> GAASMTQFEGFTNL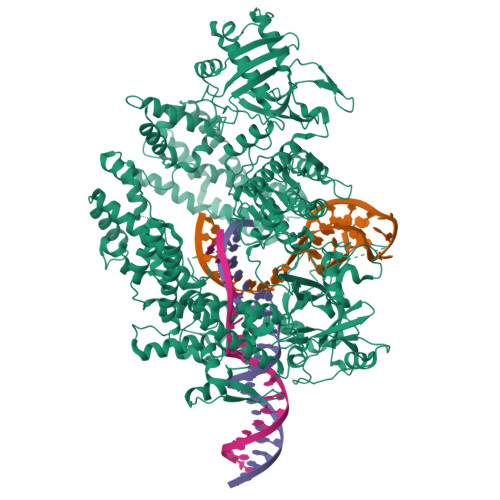YQVSKTLRFELIPQGKTLKHIQEQGFIEEDKARNDHYKELKPIIDRIYKTYADQCLQLVQLDWENLSAAIDSYRKEKTEETRNALIEEQATYRNAIHDYFIGRTDNLTDAINKRHAEIYKGLFKAELFNGKVLKQLGTVTTTEHENALLRSFDKFTTYFSGFYENRKNVFSAEDISTAIPHRIVQDNFPKFKENCHIFTRLITAVPSLREHFENVKKAIGIFVSTSIEEVFSFPFYNQLLTQTQIDLYNQLLGGISREAGTEKIKGLNEVLNLAIQKNDETAHIIASLPHRFIPLFKQILSDRNTLSFILEEFKSDEEVIQSFCKYKTLLRNENVLETAEALFNELNSIDLTHIFISHKKLETISSALCDHWDTLRNALYERRISELTGKITKSAKEKVQRSLKHEDINLQEIISAAGKELSEAFKQKTSEILSHAHAALDQPLPTTLKKQEEKEILKSQLDSLLGLYHLLDWFAVDESNEVDPEFSARLTGIKLEMEPSLSFYNKARNYATKKPYSVEKFKLNFQMPTLASGWDVNKEKNNGAILFVKNGLYYLGIMPKQKGRYKALSFEPTEKTSEGFDKMYYDYFPDAAKMIPKCSTQLKAVTAHFQTHTTPILLSNNFIEPLEITKEIYDLNNPEKEPKKFQTAYAKKTGDQKGYREALCKWIDFTRDFLSKYTKTTSIDLSSLRPSSQYKDLGEYYAELNPLLYHISFQRIAEKEIMDAVETGKLYLFQIYNKDFAKGHHGKPNLHTLYWTGLFSPENLAKTSIKLNGQAELFYRPKSRMKRMAHRLGEKMLNKKLKDQKTPIPDTLYQELYDYVNHRLSHDLSDEARALLPNVITKEVSHEIIKDRRFTSDKFFFHVPITLNYQAANSPSKFNQRVNAYLKEHPETPIIGIDRGERNLIYITVIDSTGKILEQRSLNTIQQFDYQKKLDNREKERVAARQAWSVVGTIKDLKQGYLSQVIHEIVDLMIHYQAVVVLENLNFGFKSKRTGIAEKAVYQQFEKMLIDKLNCLVLKDYPAEKVGGVLNPYQLTDQFTSFAKMGTQSGFLFYVPAPYTSKIDPLTGFVDPFVWKTIKNHESRKHFLEGFDFLHYDVKTGDFILHFKMNRNLSFQRGLPGFMPAWDIVFEKNETQFDAKGTPFIAGKRIVPVIENHRFTGRYRDLYPANELIALLEEKGIVFRDGSNILPKLLENDDSHAIDTMVALIRSVLQMRNSNAATGEDYINSPVRDLNGVCFDSRFQNPEWPMDADANGAYHIALKGQLLLNHLKESKDLKLQNGISNQDWLAYIQELRN>GPGGSPYLITGIPKDPKHPLPIRKDIDDWYLEQTSAGSNRIQLTLFVEALTVIQNRPLNDQLSYFRLAGIHGAPWTEWDGVPGGQKDSKGNPTGFAVHNNYTFPTWHRVYVTLYEQVIYEA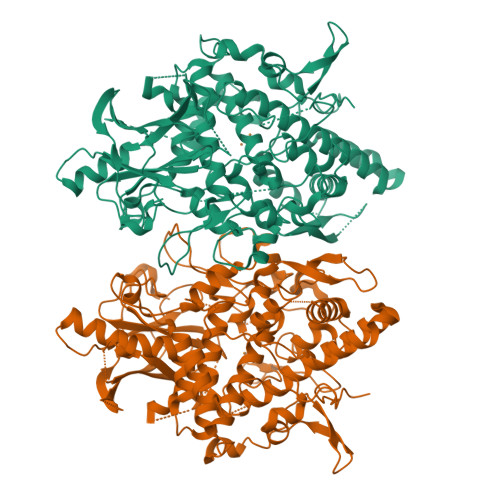MLDFIKQNVPQNGKADWENEAKQWRLPYWDFARFARHGHDNTQGDELRLPILVTMPMVKVLVPGQPGKQLSKPNPLYRFQMQTLMGTLERPYAITSQKTEEHGWSFDLPFDKCQSTTKYGLLENYNADVWADGGQNWLRANLALNEHPWYQNLDGWDSVPTLQDMTFRLLTTGGLNWGEFSSTRYDDKKEETQPKNNEQAPKNWMNLEAIHNNVHNWVGGFMFSRPGRHDLKLWGAGHMSSVPVAAYDPIFWLHHCNIDRLTAIWQTVNSGSWFNDDKSKVSKDDDLRPFHRFCEKTRKVVFFRSDDVKDWRSLNYDYAITKDASRIRKEISDLYGQRTKEVYKDFGEEDYILSIRYSRYALGGKPFQINIFFGDVDGKDFYDARSQNFVGSVFNFSGSLEDSNCDKCAQQEQEGVLSVSQLPARLAVHYYKKQNKGEVPTPRYVVVNSQGKAEAEVKVEVALHKTEGTFYDAPARGGSDDYRRVADGKRAEVDDAYRA[2x]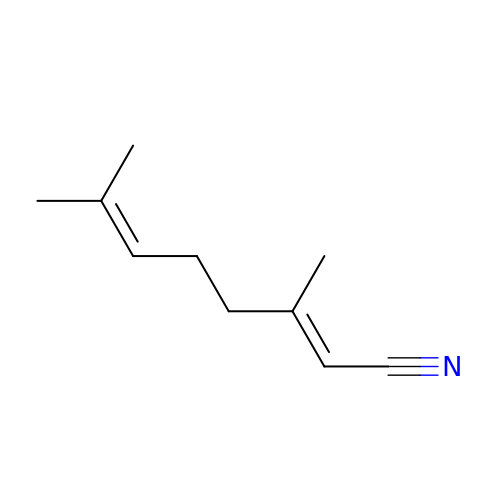(2Z)-3,7-dimethylocta-2,6-dienenitrile | C10 H15 N | HLCSDJLATUNSSI-YFHOEESVSA-N Polyomaviruses are small double-stranded DNA (dsDNA) viruses with a circular genome of approximately 5,000 bp. All glycan-binding polyomaviruses analyzed to date engage oligosaccharide (glycan) structures featuring terminal sialic acids that in mammals are usually presented either on gangliosides, which are molecules composed of a glycosphingolipid, i.e., a ceramide and an oligosaccharide, or on glycoproteins, which contain mostly complex and branched oligosaccharides attached to amino acids during co- and posttranslational modification steps. These sialylated glycan structures interact with loop regions at the outer margin of the major capsid protein VP1, at the apical surface of the polyomavirus capsid, as revealed by X-ray crystallography and cryoelectron microscopy. The VP1 surface exhibits an astonishing plasticity, providing virus-specific interactions for a range of Neu5Ac linkage types and further specific characteristics of Neu5Ac-containing glycans.

We expressed and purified assembly-incompetent VP1 pentamers from all three viruses by following the protocol established for HPyV12 and solved their crystal structures at high resolution. All three proteins fold into the familiar VP1 pentamer structure. Superpositions of the VP1 pentamers of ShPyV, GhPyV, and FiPyV with that of HPyV12 confirm that the core VP1 structure is highly conserved (RMSD values of 0.65 Å, 0.83 Å, and 0.73 Å, respectively). In HPyV12 VP1, the BC2 loop comprising the Neu5Ac-binding site is formed by amino acids T69 to Q83 (T73 to E87 in TSPyV VP1), whereas the putative binding sites in ShPyV VP1, GhPyV VP1, and FiPyV VP1 include amino acid residues T61 to Q75, T57 to E71, and T58 to E72, respectively. We calculated all-atom RMSD values with PyMOL using the BC2 loop of HPyV12 VP1 as a reference. With a value of 1.82 Å, the BC2 loop of FiPyV VP1 shows the largest deviation, while the BC2 loops of ShPyV and GhPyV VP1 yield lower deviations, of 0.77 Å and 0.84 Å, respectively. However, FiPyV did not hemagglutinate chicken or human erythrocytes, suggesting an alternative receptor specificity compared to that of the related viruses, likely influenced by residues surrounding the conserved BC2 loop Neu5Ac-binding site.

>[30x]MGSSHHHHHHSSGENLYFQGSHMGGIEVLDVKTGPDSTTTIEAYLNPRVGQNWGFSTEITVASNGYNDAPHLTEIPCYSSARISLPLLNEDITSPTLLMWEAVSVKTEVVGISSMLNMHSYGLRAFGGYGGGYTIEGSHIHFFSVGGEPLDLQGLMQNHSTQYPSPLVGPKKPDGTTDDSAQVLNPIYKAKLDKDATYPIECWCPDPSRNENSRYFGSYTGGVETPPVLSFTNTSTTILLDENGVGPLCKGDGLYLSSADVAGTFVQQTSQKQYWRGLPRYFNITLRKRAVKN> MTTYCPARGDVILLDFNPQSGHEQAGKRPALVVSDDLFNQVTGFAVVCPITNQIKGYPFEVPVDGTTKTTGVILADQVK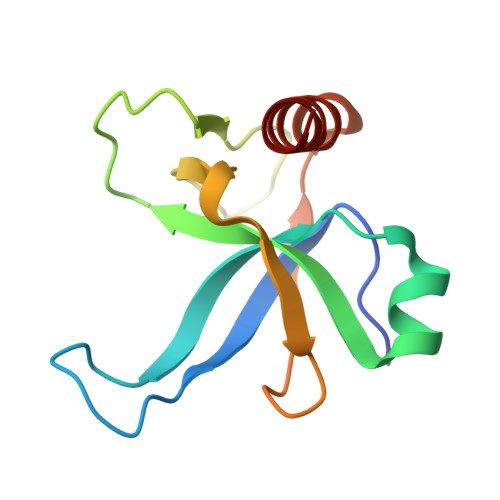SLDWKARAARTVDSVSGETVTTVVDMVSKIIKA> GEIQWVKPNKETGRLSINGPTRTKLEPSVFHDVFEGNKEPAVLHSKDPRLEVDFEQALFSKYVGNTLYEPDEYIKEAALHYANQLKQLEINTSQMSMEEACYGTENLEAIDLHTSAGYPYSALGIKKRDILDPTTRDVSKMKFYMDKYGLDLPYSTYVKDELRSIDKIKKGKSRLIEASSLNDSVYLRMAFGHLYETFHANPGTITGSAVGCNPDTFWSK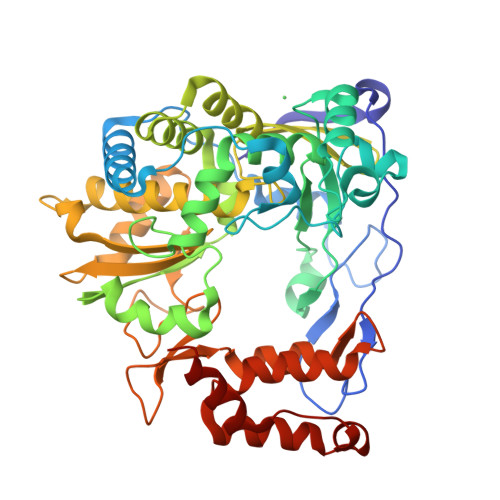LPILLPGSLFAFDYSGYDASLSPVWFRALELVLREIGYSEGAISLIEGINHTHHVYRNKTYCVLGGMPSGCSGTSIFNSMINNIIIRALLIKTFKGIDLDELNMVAYGDDVLASYPFPIDCLELAKTGKEYGLTMTPADKSPCFNEVNWDNATFLKRGFLPDEQFPFLIHPTMPMREIHESIRWTKDARNTQDHVRSLCLLAWHNGKQEYEKFVSTIRSVPVGRALAIPNYENLRRNWLELF>ALIERIDAIIVDLPTIRPHKLAMHTMQQQTLVVLRVRCSDGVEGIGEATTVGGLAYGYESPEGIKANIDAHLAPALIGLAADNINAAMLKLDKLAKGNTFAKSGIESALLDAQGKRLGLPVSELLGGRVRDSLEVAWTLASGDTARDIAEARHMLEIRRHRVFKLKIGANPVEQDLKHVVTIKRELGDSASVRVDVNQYWDESQAIRACQVLGDNGIDLIEQPISRINRGGQVRLNQRTPAPIMADESIESVEDAFSLAADGAASIFALKIAKNGGPRAVLRTAQIAEAAGIGLYGGTMLEGSIGTLASAHAFLTLRQLTWGTELFGPLLLTEEIVNEPPQY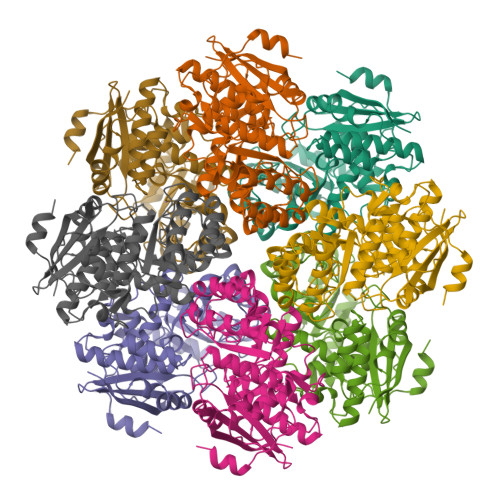RDFQLHIPRTPGLGLTLDEQRLARFAR[2x]Aldehyde dehydrogenases (ALDHs) catalyze the NAD(P)+-dependent irreversible oxidation of aliphatic and aromatic aldehydes. Human ALDH9A1 is a cytosolic tetrameric enzyme of ∼216 kDa that was first purified from the liver and characterized as a 4-aminobutyraldehyde (ABAL) dehydrogenase (ABALDH, E.C. 1.2.1.19). The enzyme is involved in the carnitine synthesis pathway comprising three other enzymes: trimethyl lysine dioxygenase, 3-hydroxy-N-trimethyllysine aldolase and γ-butyrobetaine (TMABA) dioxygenase. In the present study, using kinetic assays and affinity measurements, we showed that among various available aminoaldehydes, ALDH9A1 preferentially oxidizes TMABAL with the highest rates at very low saturating micromolar concentrations.

Co-crystallization with 50 mM NAD+ with or without 10 mM TMABA product resulted into different crystal forms. However, the three solved structures from P21212, P21, and C2 space groups at 2.5, 2.9, and 2.3 Å, respectively, reveal an ALDH9A1 apoform in the absence of a bound NAD+ or TMABA. The asymmetric units of the P21212 and P21 structures contain two similar tetramers (dimer-of-dimers) and that of C2 only one. All monomers are very similar to each other with an RMSD up to 0.24 Å. Each monomer displays the classical ALDH fold consisting of a catalytic domain (residues 258–448) with the catalytic Cys288, a coenzyme binding domain (residues 1–127, 146–257, 470–478), and an oligomerization domain (residues 128–145 and 479–494), which wraps over the groove between the catalytic and coenzyme domains of the other monomer forming the dimer. The αβE region is not visible in the electron density maps thus is highly mobile. The first one concerns the αβE region, which is composed of the α-helix E and β-strand E, located at the dimer interface. This region interacts with the bound NAD+ when present in ALDH structures, and the absence of a bound NAD+ in the HsALDH9A1 structure is in agreement with this largely disordered region. In our three HsALDH9A1 structures, the inter-domain linker adopts a unique fold, never observed so far, preventing the binding of any substrate. The same fold of the inter-domain linker in the three crystal forms suggests that this linker exhibits such conformation in the apoform. Therefore, a switch corresponding to a rearrangement up to 30 Å must occur for substrate binding followed by NAD+ binding.

>[4x]MGSSHHHHHHSQDPMSTGTFVVSQPLNYRGGARVEPADASGTEKAFEPATGRVIATFTCSGEKEVNLAVQNAKAAFKIWSQKSGMERCRILLEAARIIREREDEIATMECINNGKSIFEARLDIDISWQCLEYYAGLAASMAGEHIQLPGGSFGYTRREPLGVCVGIGAWNYPFQIASWKSAPALACGNAMVFKPSPFTPVSALLLAEIYSEAGVPPGLFNVVQGGAATGQFLCQHPDVAKVSFTGSVPTGMKIMEMSAKGIKPVTLELGGKSPLIIFSDCDMNNAVKGALMANFLTQGQVCCNGTRVFVQKEILDKFTEEVVKQTQRIKIGDPLLEDTRMGPLINRPHLERVLGFVKVAKEQGAKVLCGGDIYVPEDPKLKDGYYMRPCVLTNCRDDMTCVKEEIFGPVMSILSFDTEAEVLERANDTTFGLAAGVFTRDIQRAHRVVAELQAGTCFINNYNVSPVELPFGGYKKSGFGRENGRVTIEYYSQLKTVCVEMGDVESAF>[2x]STNDNIKDLLDWYSSGSDTFTNSEVLDNSLGSMRIKNTDGSISLIIFPSPYYSPAFTKGEKVDLNTKRTKKS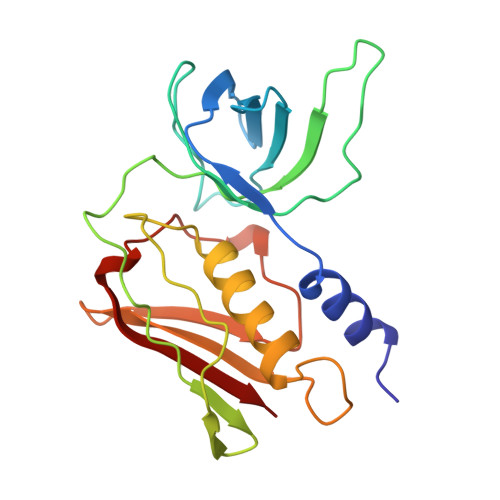QHTSEGTYIHFQISGVTNTEKLPTPIELPLKVKVHGKDSPLKYWPKFDKKQLAISTLDFEIRHQLTQIHGLYRSSDKTGGYWKITMNDGSTYQSDLSKKFEYNTEKPPINIDEIKTIEAEIN Equisetin | C22 H31 N 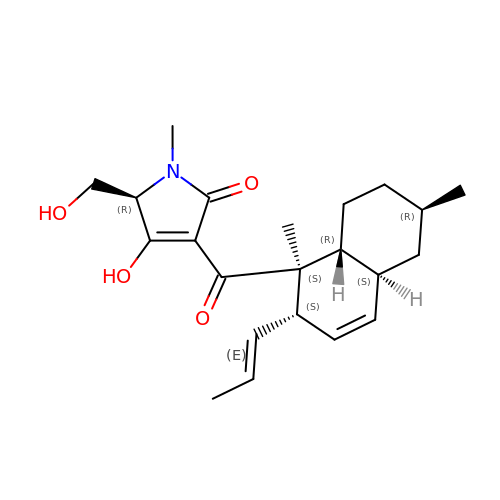O4 | YHKYFYCSTJGMID-OIKIKICYSA-N> MRKVVADLNAVEEENMPENHTPDDGHNHAHGGFLNRILGGRAEVIFAVLCGICLLLGWLGPKYGIMSEQFGFGLLLAAYFFGGYFTLREAVEKISKGQFQIDFLMLVAASGAAILGEWAEGAFLLFLFSVGHALENYAMGRARNAVAALAGLTPDEALVRRGDKTETVLIENLLVGDIVVVRSNERLPADGFVVKGSSAVNQAPITGESAPVDKLPVDDPEFAAANLDKLTPQTRVFAGSINGSGSLDVQVTKLSGESTLARVVTLVAEAQTRQSPTQNFTKKFEKIFVPCVIALAFVTSFSFLILDETAAQSFYRAMAVLVAASPCALAIATPSAVLSGVARAARGGVLIKGGAPLEAMGHLDAIAFDKTGTLTIGEPHLVEITPYGDATETELLQVSAAVEMLSDHPLAQAVVRDVKDRLGDLPSEASDFANIIGQGVSAKVDSKVVHIGKTALFESVAGLPLPDDLRGTVEAMSQNGRTTMIVRSGDRYLGAIGLMDTPREDARSVIAALRDLGLKRMMMISGDNQNVANAVAKEVGLDTAFGDLMPEDKVTKIAALKADGGVAMV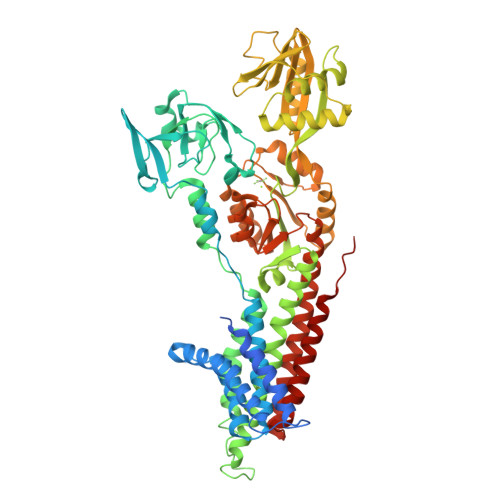GDGVNDAPAMANATVGIAMGAAGSDVALETADIALMADDLQTLPFAVGLSRKTSRIIRLNLWFSLGVVALLIPATLFGLGIGPAVLVHEGSTLVVVANALRLLAFKDNRVKSA>MKIVIVGIGYVGLANAILFSKNNENEVVLLDIDENKIQSINNHKSPIKDKLIEKFFVQNISKLHATSNIKEAYFNADFAVIATPTDYDEQLNFFDTRSIENVLKDIKNINSKINVIIKSTVPIGYTKTIKQKFNMSNIVFSPEFLREGSALYDSLYPSRIIIGDKSVLGKTIGDLFLKNIEKKNVDIFYMDSDEAESVKLFSNTYLAMRVGFFNEVDSYARKHNLNSADIIKGISADDRIGKYYNNPSFGYGGYCLPKDTK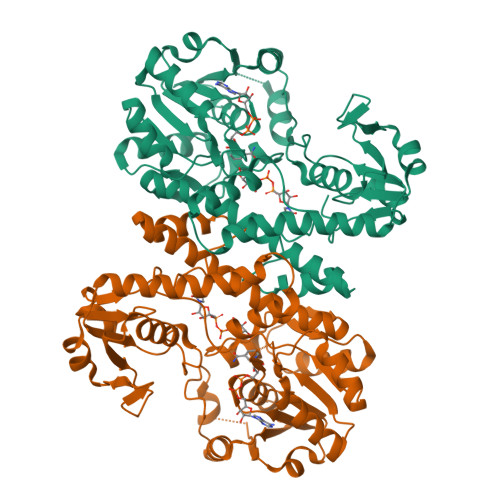QLLANFYNIPNSLIKAIVETNEIRKKFITQLILEKKPNILGIYRLIMKQNSDNFRNSVIIDIIKYLQEYNSNIELIIYEPLVKEKKFLNIKVENDFNVFGAKVDLIIANRFDDKLKEIKDKVFSADVFYTDI[2x]> SGNDDFLIPVVFPDYLISVADE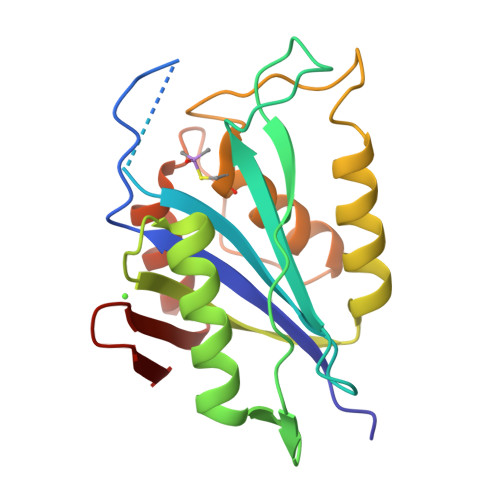QSFELWGVKIKTPAVKAPYLGHAGVILINGETGVTRYYEYGRYKNPKSDIPGNVRKVGVSNVTIKSGLITESSLLKVLKEVSLRSGQEGRISGVVLRGKFFSEADSWLRGKMDLNNSPDKIPYDLDSHNCMTFVIDLADAMGLDPAWKPPVVVPSAYIEQFQLSEIDLDYDYKTNKLTVSE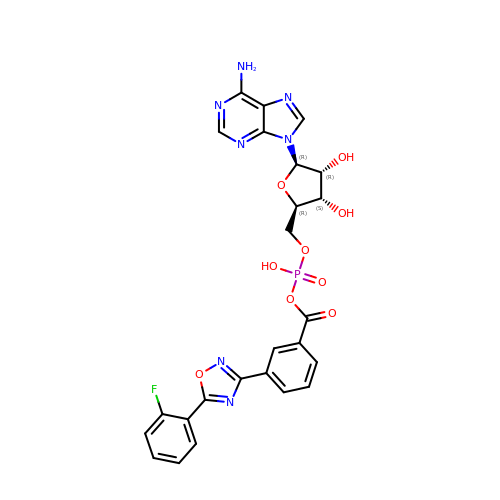5'-O-[(R)-[({3-[5-(2-fluorophenyl)-1,2,4-oxadiazol-3-yl]phenyl}carbonyl)oxy](hydroxy)phosphoryl]adenosine | C25 H21 F N7 O9 P | XGTSAMZIYGBAIU-VEBYGKHWSA-N>MRSRRVDVMDVMNRLILAMDLMNRDDALRVTGEVREYIDTVKIGYPLVLSEGMDIIAEFRKRFGCRIIADFKVADIPETNEKICRATFKAGADAIIVHGFPGADSVRACLNVAEEMGREVFLLTEMSHPGAEMFIQGAADEIARMGVDLGVKNYVGPSTRPER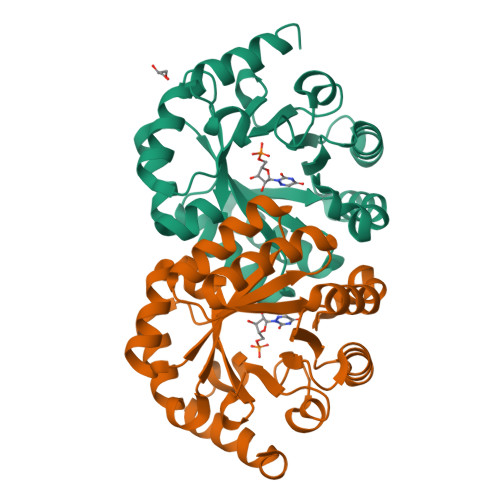LSRLREIIGQDSFLISAGVGAQGGDPGETLRFADAIIVGRSIYLADNPAAAAAGIIESIKDLLNP[2x]>EITGPYTNTIIKLSDLSGSNVWVLYQKPTSTVKLLKNGPESYSWNLAAFELWYGKANTTVTSDYYSGMTNSEKSVEVDHDSLVLFWNEGSTALSNKVINFSWNVGGVLIKLTSNTRIDVCMAD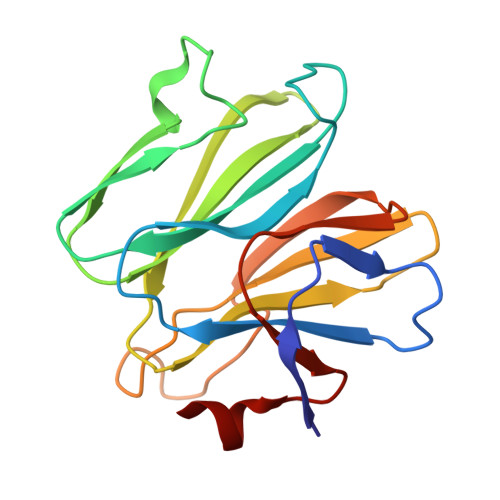MDNFTSDSFNWEEWTHNFPRSESMNIYTDYYLASVDPYSQIR[2x]> MEKTTEGAFYTREYRNLFKEFGYSEAEIQERVKDTWEQLFGDNPETKIYYEVGDDLGYLLDTGNLD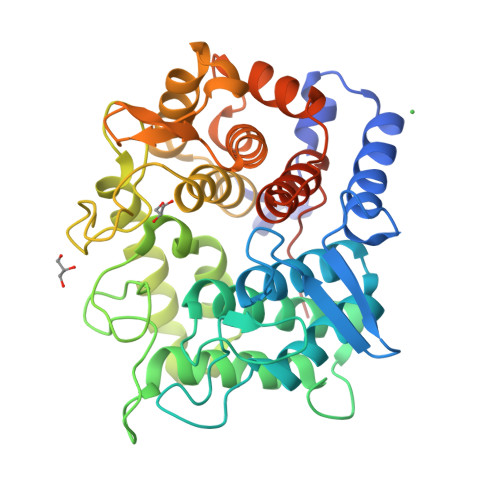VRTEGMSYGMMMAVQMDRKDIFDRIWNWTMKNMYMTEGVHAGYFAWSCQPDGTKNSWGPAPDGEEYFALALFFASHRWGDGDEQPFNYSEQARKLLHTCVHNGEGGPGHPMWNRDNKLIKFIPEVEFSDPSYHLPHFYELFSLWANEEDRVFWKEAAEASREYLKIACHPETGLAPEYAYYDGTPNDEKGYGHFFSCSYRVAANIGLDAEWFGGSEWSAEEINKIQAFFADKEPEDYRRYKIDGEPFEEKSLHPVGLIATNAMGSLASVDGPYAKANVDLFWNTPVRTGNRRYYDNCLYLFAMLALSGNFKIWFPEGQEEEHLEHHHHHH>[2x]GEMVFGKDALLGPRRPRPHKIWKKKYIKLIVVGDSGLGKTTLIKSLISIPGERLQVHDGSYTPTEQFRRDPESLSSTVSWRDEEDRVIWVYKIQDTPGYGDELDVFRNLKMVQDYIESQNRKWLELEQARDRKEDLAEIEDPRVD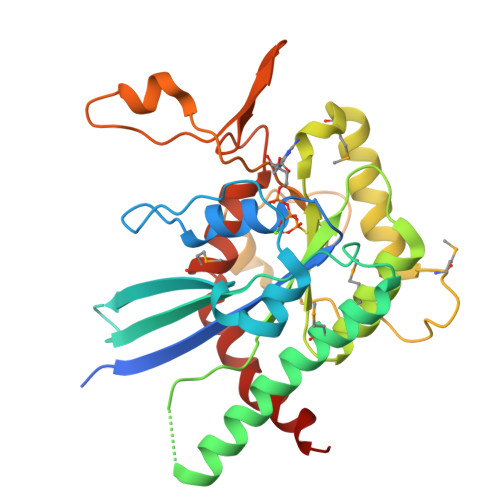LCIFCIPPHRLRPIDLKYMFELGKHVPVVPVVTKADTMTIREANTYRTEVANRIANPMVPGIHDKINIFKFERDTLERAGVQDHATPHPPFLVIASNDISEELAAAEPPLFWPERRYPWGTAEAFNKEHSDLLAVRALLMKEALEEISKTKRARYEAWRRTTL>[2x]UUAUAUAU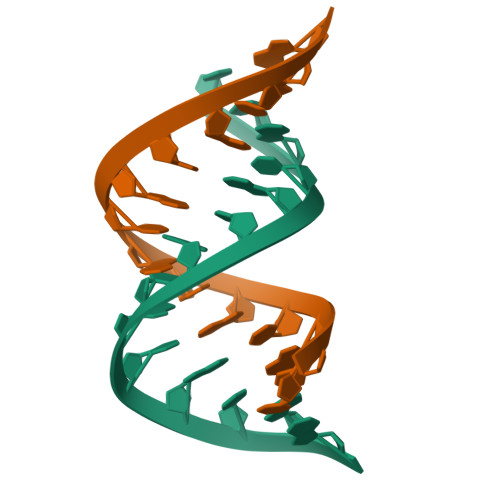AUAUAA> ACGGACACTCA;> CACACCGT;> CTGAGTGTGCTCT;> GAGAGCT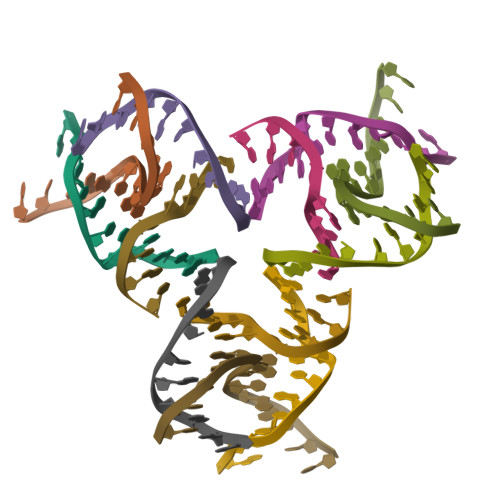GTG> MTHDNKLQVEAIKRGTVIAH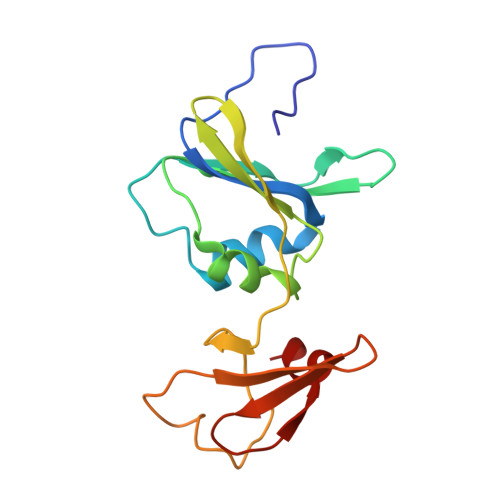IPAQIGFKLLSLFKLTETDQRITIGLNLPSGEMGRKDLIKIENTFLSEDQVDQLALYAPQATVNRIDNYEVVGKSRPSLPERIDNVLVCPNSNCISHAEPVSSSFAVRKRANDIALKCKYCEKEFSHNVVLAN> EVSIIQG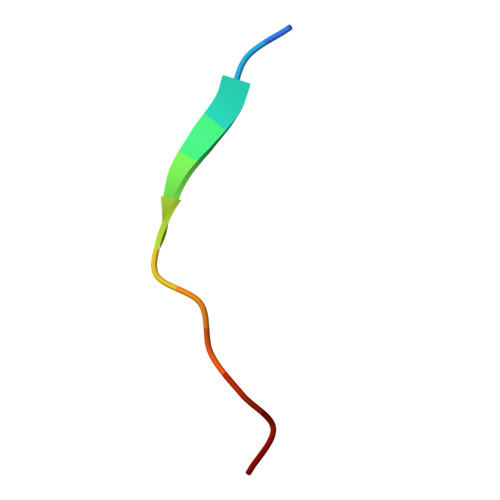ADSTT> ETAIPFSRRRMPYSLGTDKLEKVDPDKIKSKLSEDVERKLETDMRELYDRLLPTEAIEVNRRELVSKLERLFNTEWPGHDIRVHLFGSSGNLLCSDDSDVDICITTPWRELESVCMIAELLDRHGMEKVVCVSSAKVPIVKIWDPELKLACDMNVNN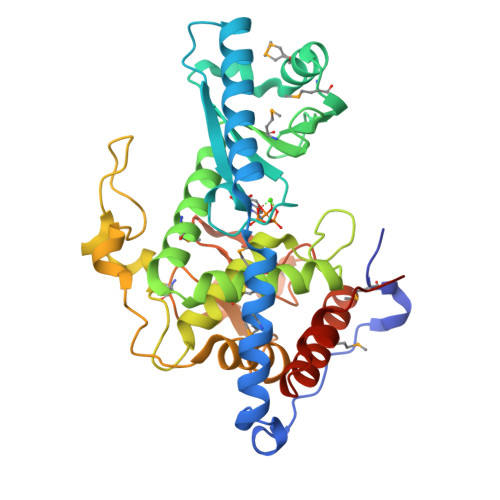TLALENTRMVRTYVSIDDRVRPLAMIIKYWTRRRVVNDAAFGGTLSSYTWICMIIAFLQLRDPPVLPALHQQHDLKLVKQDGALSDFADDIPKLRGFGAKNKDSLAVLLFQFFRFYAHEFDYDKYTLSIRMGTLLTKAEKNWQYLVNNALCVEEPFNDGRNLGNTADETSFRGLHMELRRAFDLIAEGKLEECCEQYVFPKEEERV> SMTVKEIFETMDYGPAPESAKEAYAWLAEKGDFGHFIGGAWTAPGDLFATVNPATGQTLAQVSQATQADVDAAVKAARKAQPAWAKDGAARARVLYALARLLQKHARLFAVLETLDNGKPIREARDIDVPLAQRHFYHHAGYAQLMGTEMPDRAPLGVCGQVIPWNFPLLMLAWKIAPALAMGNTVVLKPAEWTPLTALLFADICGQAGVPAGVVNIVTGDGAVGEMIVTAQVDKVAFTGSTAVGRRIREATAGTGKALSLELGGKGPYVVCDDADIDSAVEGLVDAIWFNQGQVCCAGSRLLVQEGIADVFHAKLRARMDSLRIGDPLDKCIDIGAMVHPDQLARVRDMVAANTDGEVYQTAVPAGCYYPPTLIS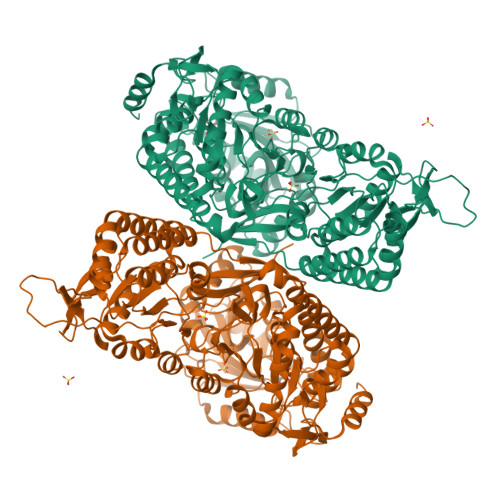GLAPASPLMQQEIFGPVLVSTTFRTPAEAVEIANNTAYGLAASVWSENVNLALDLAPKLVAGIVWINGTNMMDAAAPFGGVRESGFGREGGWEGLAGYTRPAIATKSPAAVAAYTGDGAADGLDRTAKLYIGGKQTRPDGGYSRAVYGPKGKLLGHASLSNRKDLRNAVEAMNAASGWSRTTGHLRAQILYFIGENLSARADEFANRIKDMTGKDGKAEVAASIDRLFSAAAWADKYDGQVKGVPLRGVALAMKEPVGKIGILCPDAAPLLGLVSLMAPAIAMGNRVTLAASEAFPLAATDFYQVLDTSDVPAGVVNILTGAHADLAEPMARHLDLDAVWGLSGHAQVIEAASAGNLKRSWTGPFDPAHDHTRDILSHATEVKTIWVPYGA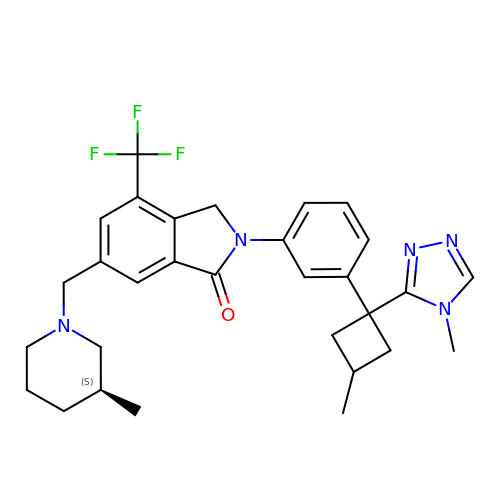2-{3-[(1s,3R)-3-methyl-1-(4-methyl-4H-1,2,4-triazol-3-yl)cyclobutyl]phenyl}-6-{[(3S)-3-methylpiperidin-1-yl]methyl}-4-(trifluoromethyl)-2,3-dihydro-1H-isoindol-1-one | C30 H34 F3 N5 O | HUOLMBXGHHSYHC-QWQFASRJSA-N> MAHHHHHHHRSSGAPAAADRGVILDLDGTLADTPAAIATITAEVLAAMGTAVSRGAILSTVGRPLPASLAGLLGVPVEDPRVAEATEEYGRRFGAHVRAAGPRLLYPGVLEGLDRLSAAGFRLAMATSKVEKAARAIAELTGLDTRLTVIAGDDSVERGKPHPDMALHVARGLGIPPERCVVIGDGVPDAEMGRAAGMTVIGVS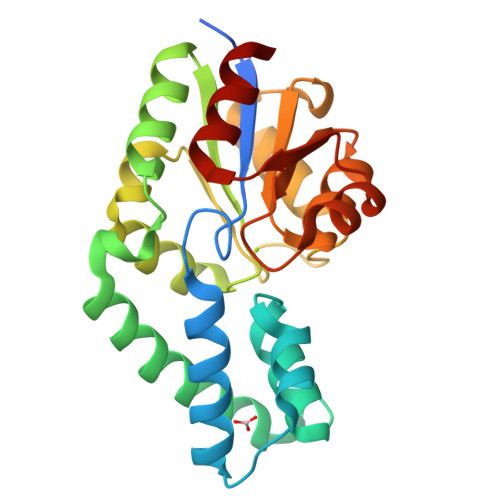YGVSGPDELMRAGADTVVDSFPAAVTAVLDGHP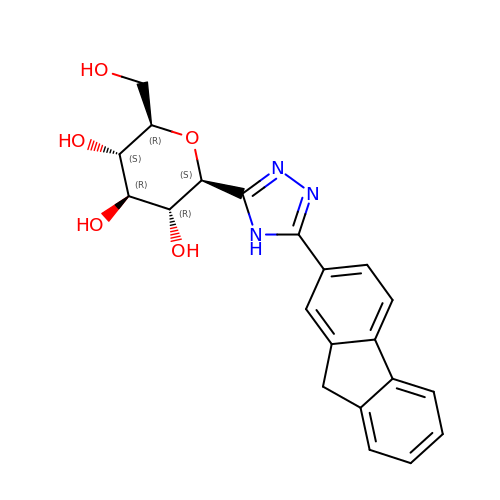(2~{S},3~{R},4~{R},5~{S},6~{R})-2-[5-(9~{H}-fluoren-2-yl)-4~{H}-1,2,4-triazol-3-yl]-6-(hydroxymethyl)oxane-3,4,5-triol | C21 H21 N3 O5 | TZDHXEVIRUMISB-UJWQCDCRSA-N> GSMTATDNARQVTIIGAGLAGTLVARLLARNGWQVNLFERRPDPRIETGARGRSINLALAERGAHALRLAGLEREVLAEAVMMRGRMVHVPGTPPNLQPYGRDDSEVIWSINRDRLNRILLDGAEAAGASIHFNLGLDSVDFARQRLTLSNVSGERLEKRFHLLIGADGCNSAVRQAMASVVDLGEHLETQPHGYKELQITPEASAQFNLEPNALHIWPHGDYMCIALPNLDRSFTVTLFLHHQSPAAQPASPSFAQLVDGHAARRFFQRQFPDLSPMLDSLEQDFEHHPTGKLATLRLTTWHVGGQAVLLGDAAHPMVPFHGQGMNCALEDAVALAEHLQSAADNAS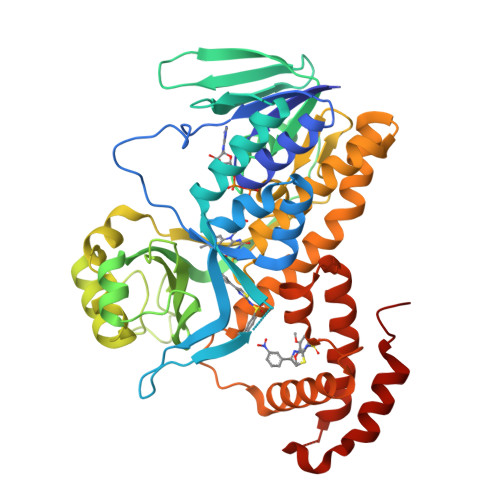ALAAFTAQRQPDALAIQAMALENYVEMSSKVASPTYLLERELGQIMAQRQPTRFIPRYSMVTFSRLPYAQAMARGQIQEQLLKFAVANHSDLTSINLDAVEHEVTRCLPPLSHLS N~6~-{N-[(1,3-dioxo-1,3-dihydro-2H-isoindol-2-yl)acetyl]-2-methyl-D-alanyl}-D-lysine | 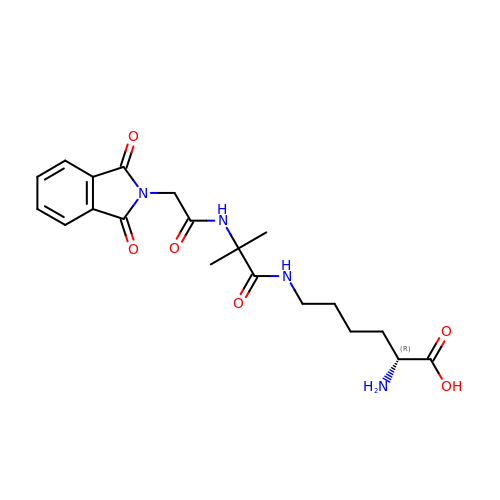C20 H26 N4 O6 | HSKHXKLBWCBTSW-CQSZACIVSA-N2-chloro-9-(3-(2,2-difluoroethoxy)benzyl)-9H-purin-6-amine | C14 H12 Cl F2 N5 O | 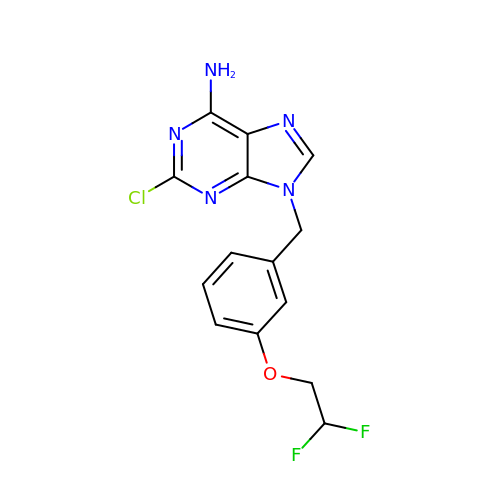SGWRECBGDPUACK-UHFFFAOYSA-N> GDTCNEETQNLSTIYLREYQSKVKRQIFSDYQSEVDIYNR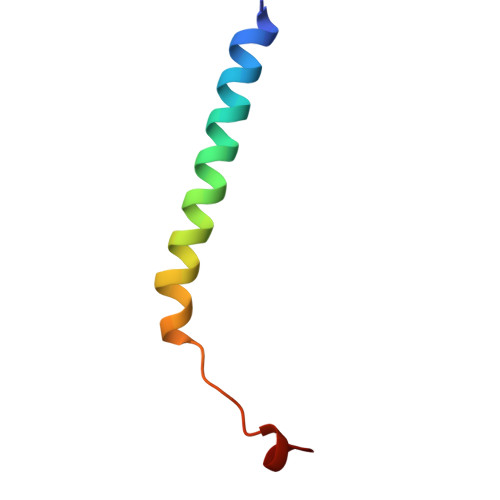I>TTCVVVRKGDEVAIGADALVTFGDTRLSRAYERNQKVIPVGDSFVGLAGTTAHFPVMRSLLTGMGEECRLHTRDDVFRTFLKVHEKLKNEYFINTKEDEDDPYESSQIVCLIANSGGIFGVYSYREVFSFDRFWG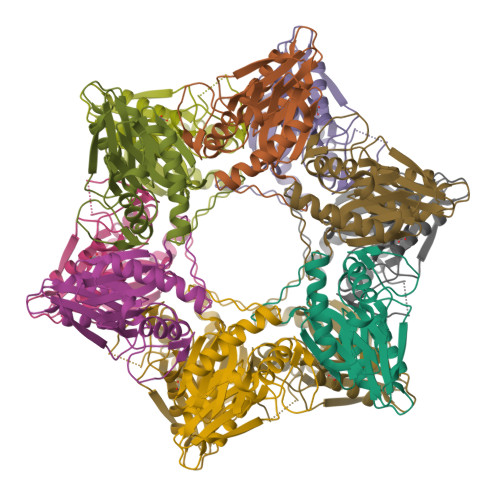IGSGRNYALGAMHAVYDRTDLDAGAIARIGVEAGIEFDKSSAAPIDVHTVRLQVATNKDGAA[2x]> GHDCHLSDMLQQLHSVNASKPSERGLVRQEEAEDPACIPIFWVSKWVDYSDKYGLGYQLCDNSVGVLFNDSTRLILYNDGDSLQYIERDGTESYLTVSSHPNSLMKKITLLKYFRNYMSEHLLKAGANITPREGDELARL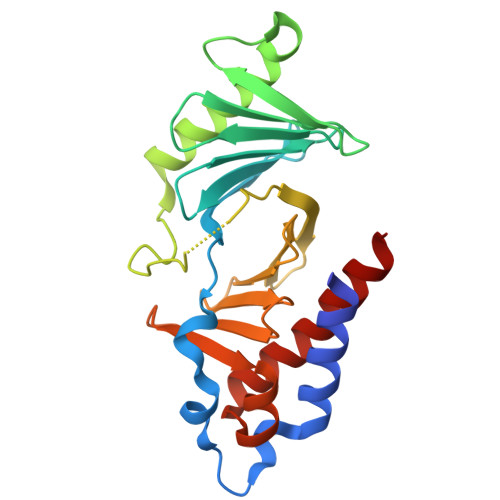PYLRTWFRTRSAIILHLSNGSVQINFFQDHTKLILCPLMAAVTYIDEKRDFRTYRLSLLEEYGCCKELASRLRYARTMVDKLLSSR>[8x]PLHHLMIGTWTPPGAIFTVQFDDEKLTCKLIKRTEIPQDEPISWMTFDHERKNIYGAAMKKWSSFAVKSPTEIVHEASHPIGGHPRANDADTNTRAIFLLAAKQPPYAVYANPFYKFAGYGNVFSVSETGKLEKNVQNYEYQENTGIHGMVFDPTETYLYSADLTANKLWTHRK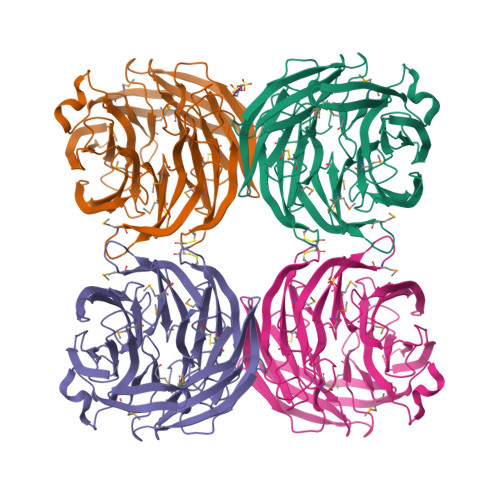LASGEVELVGSVDAPDPGDHPRWVAMHPTGNYLYALMEAGNRICEYVIDPATHMPVYTHHSFPLIPPGIPDRDPETGKGLYRADVCALTFSGKYMFASSRANKFELQGYIAGFKLRDCGSIEKQLFLSPTPTSGGHSNAVSPCPWSDEWMAITDDQEGWLEIYRWKDEFLHRVARVRIPEPGFGMNAIWYD>CGTATACG[2x]

In this study, we used d(CGTATACG)2, which forms a tetraplex base-pair junction that resembles the DNA–DNA contact structure, as a model target for two alkyl-linked diaminoacridine bis-intercalators, DA4 and DA5. To explore the possibility of targeting inter-DNA duplex structures, we synthesized two acridine-based derivatives, DA4 and DA5, by coupling 9-aminoacridine moieties with hydrocarbon chains of four and five atoms, respectively. Cross-linking of the junction site by the bis-intercalators induced substantial structural changes in the DNA, transforming it from a B-form helical end-to-end junction to an over-wounded side-by-side inter-duplex conformation with A-DNA characteristics and curvature. Furthermore, we have shown that the different topological changes induced by DA4 and DA5 lead to the inhibition of topoisomerase 2 activities, which may account for their antitumor effects.

To understand the basis for crossover structure formation at two DNA interfaces, we used a d(CGTATACG)2 DNA with terminal CG sites flanked by AT-rich sequences as a model and determined its crystal structure in P41212 space group at a resolution of 2.70 Å. The structure assembly of this complex featured symmetry related identical intertwined right-handed duplexes. These duplexes formed a helix–helix junction at the terminal C–G base pairs. Detailed analysis of this structure revealed that the distortion of the terminal C–G base pairs created a cavity that accommodates the ends of another duplex, forming a right-handed helix–helix junction structure with two duplexes in close proximity. The interface of this junction consisted of a two-layered arrangement of four-stranded base pairs. The first tetraplex base pairing was formed between C7*–G10* Watson–Crick base pairing of one duplex and the terminal bases C1 and G16 of the other duplex. Similarly, the second tetraplex base pairing was formed between the G2–C15 Watson–Crick base pairing of one duplex and the terminal G8* and C9* bases of the other duplex. This feature partially resembles the crossover sites containing DNA–DNA contact structure in catenated DNA. In the DNA-alone structure, the terminal base pairs C1–G16 and G8–C9 exhibited an unexpected distortion, failing to form a standard base pair. Instead, the cytosine bases (C1 and C9) protruded away from the helical axis, whereas the complementary guanines (G8 and G16) adopted a highly distorted extrahelical conformation with their Hoogsteen edges aligned outside the helical axis.>NKNNDKLTLWTTPDTSPNCRIDQDKDSKLTLVLTKCGSQILANVSLIVVAGRYKIINNNTNPALKGFTIKLLFDKNGV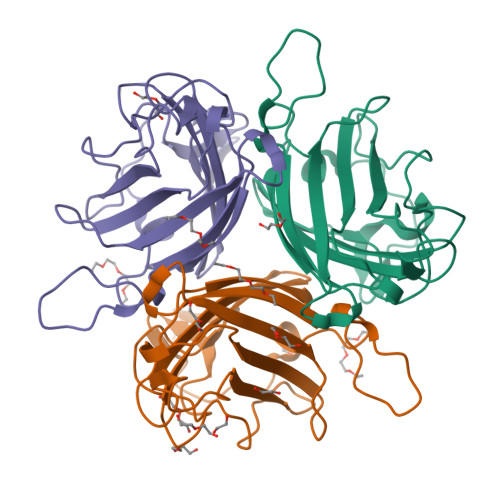LMESSNLGKSYWNFRNQNSIMSTAYEKAIGFMPNLVAYPKPTTGSKKYARDIVYGNIYLGGKPHQPVTIKTTFNQETGCEYSITFDFSWAKTYVNVEFETTSFTFSYIAQE[12x]>AETVESCLAKPHTENSFTNVWKDDKTLDRYANYEGCLWNATGVVVCTGDETQCYGTWVPIGLAIPENEGGGSEGGGSEGGGSEGGGTKPPEYGDTPIPGYTYINPLDGTYPPGTEQNPANPNPSLEESQPLNTFMFQNNRFRNRQGALTVYTGTVTQGTDPVKTYYQYTPVSSKAMYDAYWNGKFRDCAFHSGFNEDPFVCEYQGQSSDLPQPPVNAGGGSGGGSGGGSEGGGSEGGGSEGGGSEGGGSGGGSGSGDFDYEKMANANKGAMTENADENALQSDAKGKLDSVATDYGAAIDGFIGDVSGLANGNGATGDFAGSNSQMAQVGDGDNSPLMNNFRQYLPSLPQSVECRPFVFGAGKPYEFSIDCDKINLFRGVFAFLLYVATFMYVFSTFANILRNKES[5x];>AEGDDPAKAAFNSLQASATEYIGYAWAMVVVIVGATIGIKLFKKFTSKAS[15x];>MPVLLGIPLLLRFLGFLLVTLFGYLLTFLKKGFGKIAIAISLFLALII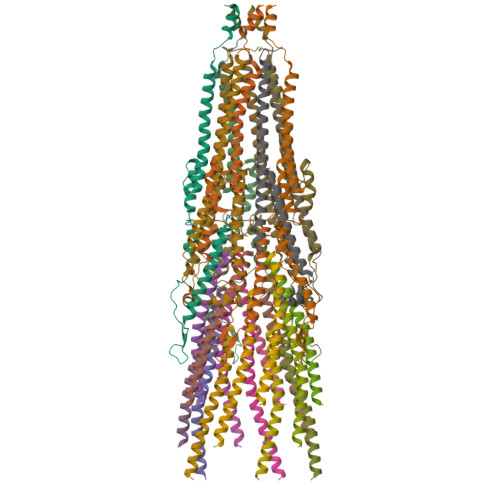GLNSILVGYLSDISAQLPSDFVQGVQLILPSNALPCFYVILSVKAAIFIFDVKQKIVSYLDWDK[5x]> MSSAFSGLKIPELSVDPAEVFKSDNPQLVSVLLDEFELQEQRPFFSGLIPEKQINIALKKSPQLKKLACHLLEAYEI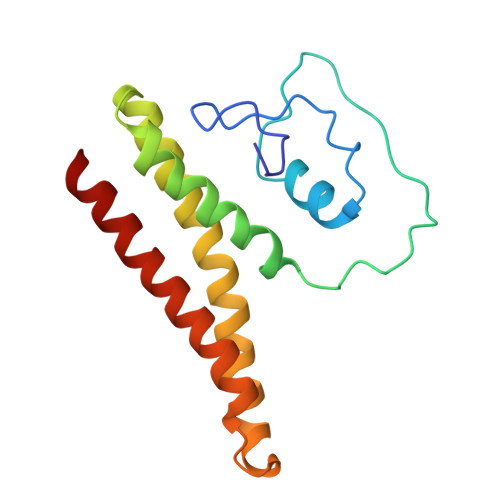NGRRWKHADRRRVLEKAIRLLEKVSNELKGDIQKLENNVKESGKDSEELNKTREKHGEILADMGRAYLHRAKII> GPDSMVPVKKEWAHVVDLNHKIENFDELIPNPARSWPFELDTFQKEAVYHLEQGDSVFVAAHTSAGKTVVAEYAIAMAHRNMTKTIYTSPIKALSNQKFRDFKETFDDVNIGLITGDVQINPDANCLIMTTEILRSMLYRGADLIRDVEFVIFDEVHYVNDQDRGVVWEEVIIMLPQHVKFILLSATVPNTYEFANWIGRTKQKNIYVISTPKRPVPLEINIWAKKELIPVINQNSEFLEANFRKHKEILNGESAKGAPSKTDNGRGGSTARGGRGGSNTRDGRGGRGNSTRGGANRGGSRGAGAIGSNKRKFFTQDGPSKKTWPEIVNYLRKRELLPMVVFVFSKKRCEEYADWLEGINFCNNKEKSQIHMFI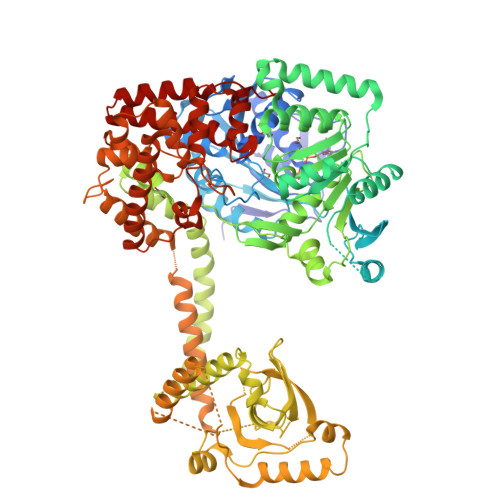EKSITRLKKEDRDLPQILKTRSLLERGIAVHHGGLLPIVKELIEILFSKGFIKVLFATETFAMGLNLPTRTVIFSSIRKHDGNGLRELTPGEFTQMAGRAGRRGLDSTGTVIVMAYNSPLSIATFKEVTMGVPTRLQSQFRLTYNMILNLLRIEALRVEEMIKYSFSENAKETLQPEHEKQIKVLQEELQTIEYKSCEICDNDIEKFLELMLAYKEATVNLMQEMVKSPSILHILKEGRLVAFRDPNDCLKLGFVFKVSLKDAVCVIMTFTKPYKLPNGEPNHLIYFPKADGYRRRNFPKFQKTDFYMEEVPVTAIEVITKRKFAAPLGKVIKKDVAALNEFNAETNNILDGKTLKEAINIEKQGLKIHQILLDRTNIRDEIFKLKSIKCPNLSQHIVPKFKAHVIKKKIEELYHLMSDQNLSLLPDYEKRLAVLKDTEFIDQNHNVLLKGRVACEINSGYELVLTELILDNFLGSFEPEEIVALLSVFVYEGKTREEEPPIVTPRLAKGKQRIEEIYKKMLCVFNTHQIPLTQDEAEFLDRKRFAMMNVVYEWARGLSFKEIMEMSPEAEGTVVRVITWLDEICREVKTASIIIGNSTLHMKMSRAQELIKRDIVFAASLYL>[2x]APVPTYQTLIVRPGDLQQSVLATGKLDALRKVDVGAQVSGQLKTLSVAIGDKVKKDQLLGVIDPEQAENQIKEVEATLMELRAQRQQAEAELKLARVTYSRQQRLAQTQAVSQQDLDNAATEMAVKQAQIGTIDAQIKRNQASLDTAKTNLDYTRIVAPMAGEVTQITTLQGQTVIAAQQAPNILTL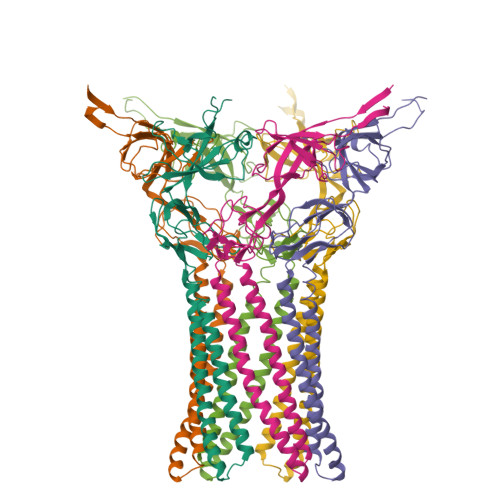ADMSAMLVKAQVSEADVIHLKPGQKAWFTVLGDQLTRYEGQIKDVLPTPEKVNDAIFYYARFEVPNPNGLLRLDMTAQVHIQLTDVKNVLTIPLSALGDPVGDNRYKVKLLRNGETREREVTIGARNDTDVEIVKGLEAGDEVVIGEAKPGAAQ>ANSKEVKKRASSFEWFGSNESGAEFGSGNIPGVEGTDYTFPNTTAIQILIDAGMNIFRVPFLMERMIPTEMTGSLDTAYFEGYSEVINYITGKGAHAVVDPHNFGRYYGTPISSTSDFQTFWS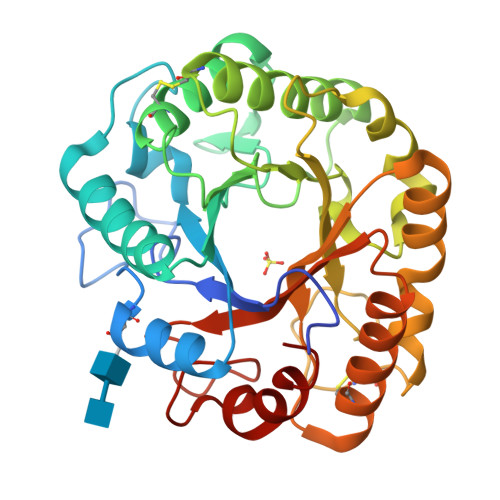TLACQFKSNDLVIFDTNNEYHDMDESVVVALNQAAIDGIRDCGATTQYIFVEGNAYSGAWTWTTYNTAMVNLTDPSDLIVYEMHQYLDSDGSGTSDQCVSSTVGQERVVDATTWLQSNGKLGILGEFAGGANSVCEEAVEGMLDYLAENSDVWLGASWWSAGPWWQDYIYSMEPPNGIAYESYLSILETYF[4x]> TASTEM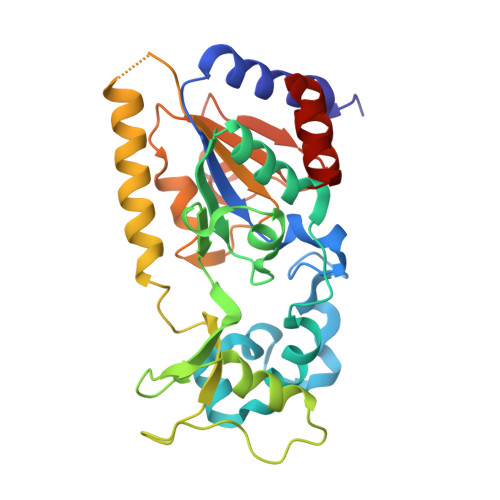SVRKIAAHMKSNPNAKVIFMVGAGISTSCGIPDFRSPGTGLYHNLARLKLPYPEAVFDVDFFQSDPLPFYTLAKELYPGNFRPSKFHYLLKLFQDKDVLKRVYTQNIDTLERQAGVKDDLIIEAHGSFAHCHCIGCGKVYPPQVFKSKLAEHPIKDFVKCDVCGELVKPAIVFFGEDLPDSFSETWLNDSEWLREKITTSGKHPQQPLVIVVGTSLAVYPFASLPEEIPRKVKRVLCNLETVGDFKANKRPTDLIVHQYSDEFAEQLVEELGWQEDFEKILTA> MMGYIP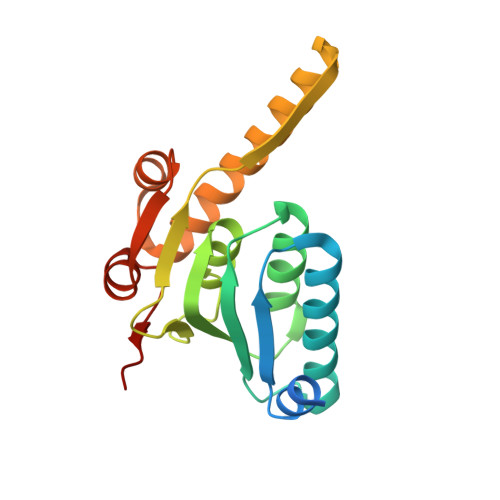YVIENTDRGERSYDIYSRLLKDRIVLLSGEINDSVASSIVAQLLFLEAEDPEKDIGLYINSPGGVITSGLSIYDTMNFIRPDVSTICIGQAASMGAFLLSCGAKGKRFSLPHSRIMIHQPLGGAQGQASDIEIISNEILRLKGLMNSILAQNSGQSLEQIAKDTDRDFYMSAKEAKEYGLIDKVLQKNVK> TETTSFSITKFSPDQQNLIFQGDGYTTKGKLTLTKAVKSTVGRALYSTPIHIWDRDTGNVANFVTSFTFV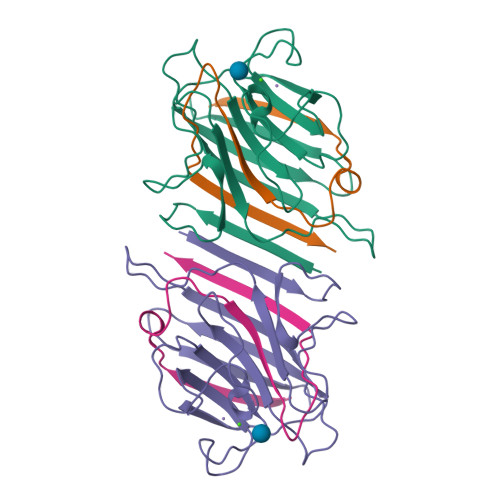IDAPSSYNVADGFTFFIAPVDTKPQTGGGYLGVFNSKEYDKTSQTVAVEFDTFYNAAWDPSNKERHIGIDVNSIKSVNTKSWNLQNGERANVVIAFNAATNVLTVTLTYPN;> VTSYTLNEVVPLKDVVPEWVRIGFSATTGAEFAAQEVHSWSFNSQLGHTSKS A HEPN (higher eukaryote and prokaryote nucleotide binding) nuclease Las1 and a polynucleotide kinase Grc3 assemble into a tetramerase responsible for rRNA maturation. Las1 and Grc3 are highly conserved proteins and have recently been identified as core enzymes involved in processing and removing ITS2 spacer, which is a key step in the synthesis of 60S ribosomal subunit. Recent studies have demonstrated that Las1 is an endoribonuclease that contains a HEPN (higher eukaryote and prokaryote nucleotide binding) domain responsible for rRNA processing. Grc3 is a polynucleotide kinase responsible not only for Las1 nuclease activation, but also for nonspecific phosphorylation of the 5′-OH of the 26S pre-rRNA produced by Las1 cleavage, providing a signal for further processing by Rat1-Rai1 exonuclease.

Cleavage assay indicates that ScGrc3 can activate ScLas1 nuclease well for ITS2 cleavage, while CjGrc3 exhibits relatively weak activation ability for CjLas1 nuclease. To better understand the differences in the mechanisms of Grc3 activation of Las1 between different species, we also solved the cryo-EM and crystal structures of full-length CjLas1-Grc3 complex at 3.39 Å and 3.39 Å resolution, respectively. Since the crystal structures have similar quality and resolve more structural information than the cryo-EM structures, the subsequent presentations and descriptions are based more on the crystal structures. Structural superposition shows that the conformations of all Grc3 domains and Las1 HEPN domains are almost identical in the two complexes, while the conformations of Las1 CC domains are significantly different. We compared the HEPN domain dimer structures in CjLas1 and CjLas1-Grc3 complex by superposition and observed that significant conformational changes occur in HEPN domains upon Grc3 binding. In the Grc3-free Las1 structure, the catalytic residues Arg129, His130, and His134 within one HEPN domain are far from the catalytic residues in the other HEPN domain, while in the Grc3-bound structure, the catalytic residues within two HEPN domains are close to each other. Notably, compared with CjGrc3-bound CjLas1, ScGrc3-bound ScLas1 has a more compact catalytic pocket, which may explain why ScLas1 shows better ITS2 cleavage activity than CjLas1 in the presence of Grc3. In addition, His130 in the ScLas1-Grc3 complex active site and the analogous His130 in the CjLas1-Grc3 complex active site adopt two different conformations, which are similar to the conformations of His142 of CtGrc3-bound CtLas1 in two different active states. This observation may also provide a structural rationale for the activation of ScLas1 and CtLas1 by Grc3, as well as for the fairly weak activation of CjLas1 by CjGrc3.

>[3x]MHKSAFQALQGDIPTYEVNSSDEQDSDQDEEDVEQPSEPMHRLVSAPAASIHIEESKYISSNFSFDDDNTIYGHDYVIFGLKSNQNLIVKGQFVLEIQRGAIDINGVIYHSGVEPMKFINPSSSSIPLIQATQVLNSSLLENKESQENQHLFTPGYKSVIKLTNLDTHLESIGRVCPLFKNLFWQFDNFFAEDSLRLLDQYELAFSDYTFYPITKPDNTVSVIKHKNWMDVIKSLTELYSNDQSIKVIVIGGKNSGKSTFLRLLVQHMLSPTLQQLPINFMDLDPGQPEYSGTDCISLSKISEVQHGNHLSLTSTDSTQCHYVGFNSPKDQPTRYNLLVEQLVRSYESDGELKHESLLINTPGWIKGYGLELTRTLIERVKPTHVIYLNSGTLGVDIDIPKGTNLIPLQGSFNHSGSRYSSSQLRLLKTMAYFHKIDDFKFDFQPLLFSPPIQVSYGVSTGISALTHLKETGIGMDHLERSIEATIVGIFKVKRDHLEECELFNKGQLPLLPYKEFIKLSTEFFRLALVHSIDQEKKIMNLYIPQFRTLDLTKEAIIMVRGNTDLPIWEIASNEIVKRFKRQLPYITFEKGSSLEKKWKVRKNVQRRGQM;>MNSHPRLTPWKSSDEVVYLKGLFFPADREQISRDELYRQYEEAISLVEMYSSRTRVSHILQSTAHLFSALMMLESFEGGLDDTVRLTASMTIIRFVNGLLDPNQQSQFAIPLHLLAKKIDLPSLFVEFRHSATHDALPSLEMCKTCVDRAIDWVWDHYWDGVLSIVEPQVETDDLEESLIKELKDLFKQYRRIRRQNITKLYKFGDSTPEGKEYWTCIAGIKDHADMANFYNVMIERIVSNKLKWEHLRALFEPMMNHFIHLKGWDFPLGLIDSMLSKNYEYSKFRGIDDTERAYLNDQEFKCAQKWIRWLAIEQIDRYDDVLVSKMIDTLGKTNHELNVELLEKLQSRFSADPVIKDKIQAKLTLIQRLSTDTKTKRMNNLEDIMSDLESLKKRAKVTPTLHIKSFESHPNWTPKPFGVI[3x]> MVDGNYSVASNVMVPMRDGVRLAVDLYRPDADGPVPVLLVRNPYDKFDVFAWSTQSTNWLEFVRDGYAVVIQDTRGLFASEGEFVPHVDDEADAEDTLSWILEQAWCDGNVGMFGVAYLGVTQWQAAVSGVGGLKAIAPSMASADLYRAPWYGPGGALSVEALLGWSALIGTGLITSRSDARPEDAADFVQLAAILNDVAGAASVTPLAEQPLLGRLIPWVIDQVVDHPDNDESWQSISLFERLGGLATPALITAGWYDGFVGESLRTFVAVKDNADARLVVGPWSHSNLTGRNADRKFGIAATYPIQEATTMHKAFFDRHLRGETDALAGVPKVRLFVMGIDEWRDETDWPLPDTAYTPFYLGGSGAANTSTGGGTLSTSISGTESADTYLYDPADPVPSLGGTLLFHNGDNGPADQRPIHDRDDVLCYSTEVLTDPVEVTGTVSARL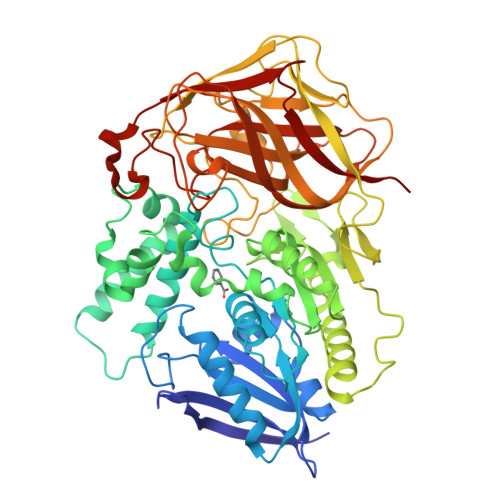FVSSSAVDTDFTAKLVDVFPDGRAIALCDGIVRMRYRETLVNPTLIEAGEIYEVAIDMLATSNVFLPGHRIMVQVSSSNFPKYDRNSNTGGVIAREQLEEMCTAVNRIHRGPEHPSHIVLPIIKR> KTNIIE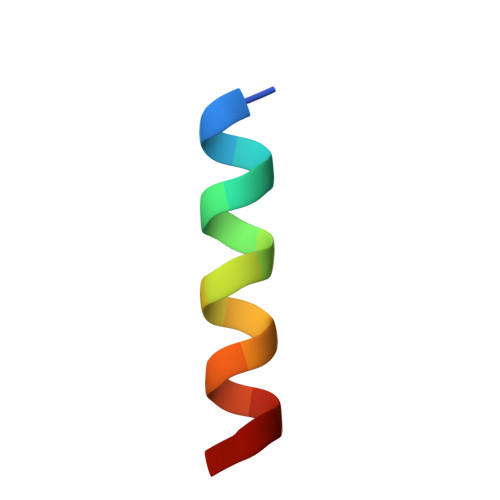KAMDYAISIEN>[4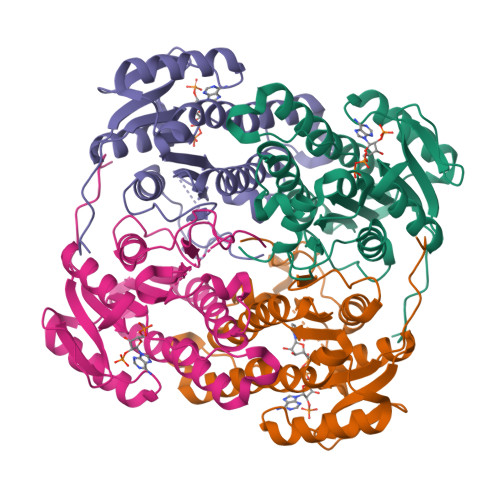x]GMTVTDNPADTAGEATAGRPAFVSRSVLVTGGNRGIGLAIARRLAADGHKVAVTHRGSGAPDDLFGVQCDVTDSAAVDRAFKEVEEHQGPVEVLVANAGISKDAFLMRMTEERFEEVINTNLTGAFRCAQRASRTMQRKRFGRIIFIGSVSGMWGIGNQANYAAAKAGLIGMARSISRELAKAGVTANVVAPGYIDTEMTRALDERIQAGALDFIPAKRVGTAEEVAGAVSFLASEDASYIAGAVIPVDGGMGMGH> MAISLATKAATNRAPVGVEPQEVHKWLQSFNWDFKENRTKYPTKYHMANETKEQFKVIAKEYARMEAAKDERQFGTLLDGLTRLGAGNKVHPRWGETMKVISNFLEVGEYNAIAASAMLWDSATAAEQKNGYLAQVLDEIRHTHQCAFINHYYSKHYHDPAGHNDARRTRAIGPLWKGMKRVFADGFISGDAVECSVNLQLVGEACFTNPLIVAVTEWASANGDEITPTVFLSVETDELRHMANGYQTVVSIANDPASAKFLNTDLNNAFWTQQKYFTPVLGYLFEYGSKFKVE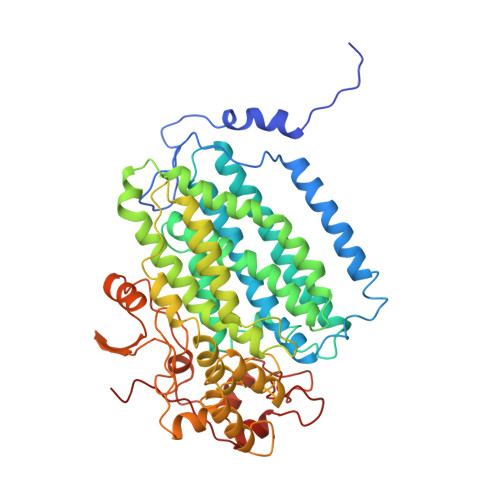PWVKTWNRWVSEDWGGIWIGRLGKYGVESPRSLRDAKRDAYWAHHDLALAAYAMWPLGFARLALPDEEDQAWFEANYPGWADHYGKIFNEWKKLGYEDPKSGFIPYQWLLANGHDVYIDRVSQVPFIPSLAKGTGSLRVHEFNGKKHSLTDDWGERQWLIEPERYECHNVFEQYEGRELSEVIAEGHGVRSDGKTLIAQPHTRGDNLWTLEDIKRAGCVFPDPLAKF> HGEKSQQAFLRMRTLNWYDVKWSKTSLNVNESMVLSGKVHVFSAWPQAVANPKSSFLNAGEPGPVLVRTAQFIGEQFAPRSVSLEVGKDYAFSIDLKARRAGRWHVHAQINVEGGGPIIGPGQWIEIKGDMADFKDPVTLLDGTTVDLETYGIDRIYAWHFPWMIAAAAWILYWFFKKGIIASYLRISEGKDEEQIGDDDRRVGAIVLAVTILATIIGYAVTNSTFPRTIPLQAGLQKPLTPIIEEGTAGVGPHVVTAELKGGVYKVPGRELTIQVKVTNKTDEPLKLGEYTAAGLRFLNPDVFTTKPEFPDYLLADRGLSTDPTPLAPGETKTIEVKVQDARWDIERLSDLAYDTDSQIGGLLMFFSPSGKRYATEIGGPVI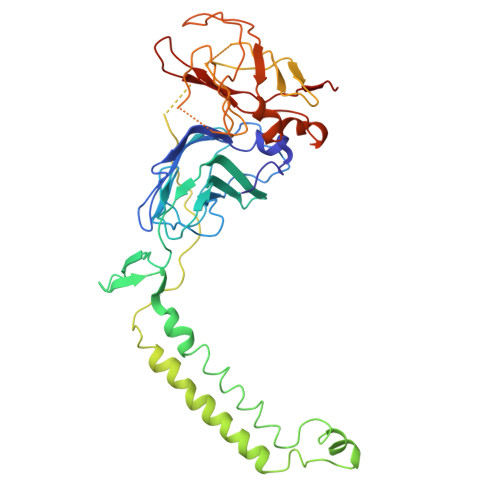PKFVAGDMP> ALLRQAYSALFRRTSTFALTVVLGAVLFERAFDQGADAIFEHLNEGKLWKHIKH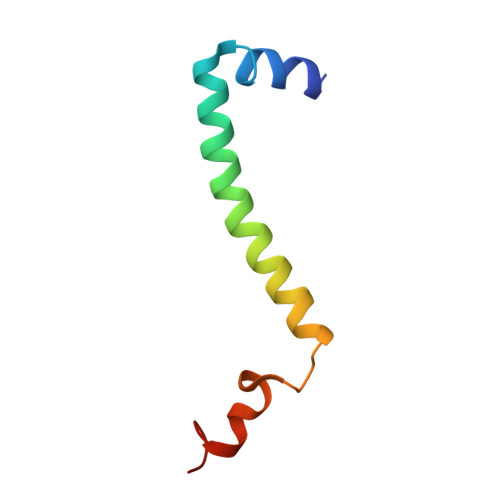KYEASEE> MAYDLSEFMGDIVALVDKRWAGIHDIEHLANAFSLPTPEIKVRFYQDLKRMFRLFPLGVFSDE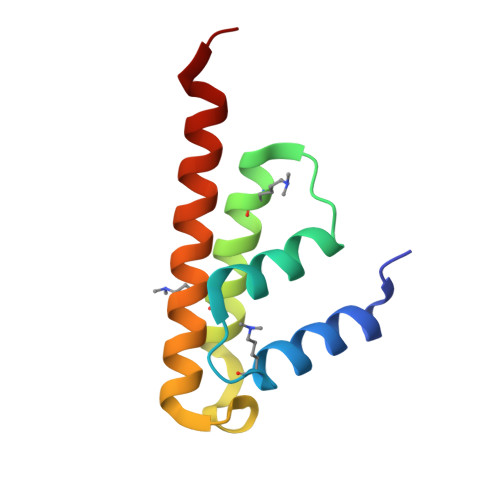EQRQNLLQMCQNAIDMAIESEEEELSELD>[4x]MNTKIKVAIVGYGNIGRFALEAVQAAQDFELVGVVRRDINNVPEELQNITVTNDIKTLGDVDVALLCSPTRAIKELAKSILSLGINTVDSFDVHSEIVSLKTELDDVAKKHDRVAVISAGWDPGSDSIVRTLMLAMAPKGITYTNFGPGMSMGHSVAAKAIEGVKDALSMTIPLGTGVHRRMVYVELEAGANFNQVEQAIKADSYFSSDETHVKQVDSVDSLKDVGHGVHMTHKGVSGKTHNQ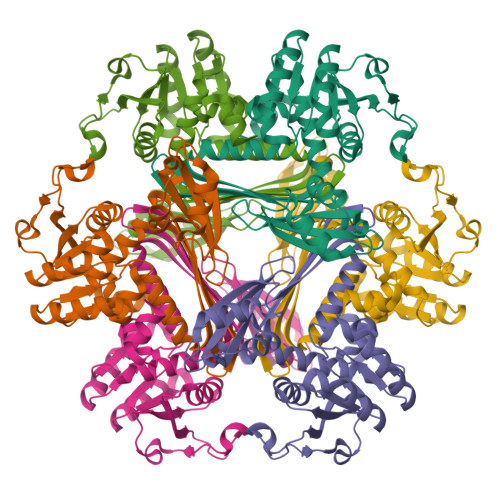LFEYSMRINNPALTSQFMVSAARASMKQRAGAYTVIEIPPVDFLAGDLNTLIAKLV>[2x]HHHHHHFNLPPGNYKKPKLLYCSNGGHFLRILPDGTVDGTRDRSDQHIQLQLSAESVGEVYIKSTETGQYLAMDTDGLLYGSQTPN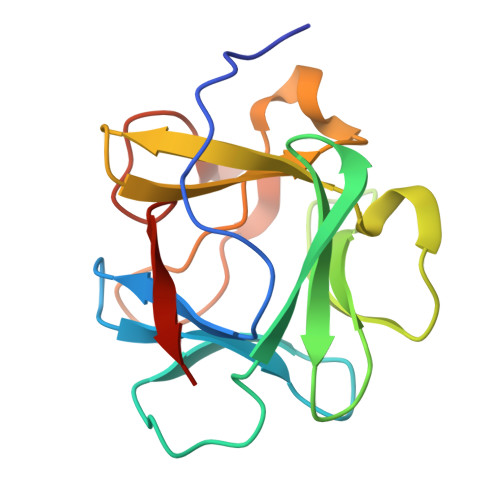EECLFLERLEENHYNTYISKKHAEKNWFVGLNKAGSCKRGPRTHYGQKAILFLPLPVSSD>[2x]SHMQPFVYMAAPARIVFSAGSSADVAEEIRRLGLSRALVLSTPQQKGDAEALASRLGRLAAGVFSEAAMHTPVEVTKTAVEAYRAAGADCVVSLGGGSTTGLGKAIALRTDAAQIVIPTTYAGSEVTPILGQTENGVKTTMRGPEILPEVVIYDAELTLGLPVAISMTSGLNAMAHAAEALYARDRNPIASMMAVEGL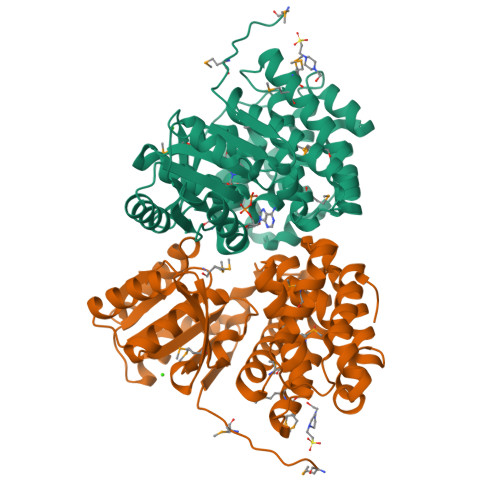RAMIEALPVVRQAPHDIGARETALYGAWLCGTVLGAVGMSLHHKLCHTLGGSLDLPHAETHAVLLPHTIAYVEEAAPNLLAPLAALVGGRAGAGLFDFAARLGAPSSLAALGVGADDLDPMAELATANPYWCPRPIEKTAIRDLLQRAFEGARPA> GPMTSQKLVRLPGLIDVHVHLREPGGTHKEDFASGTAAALAGGITMVCAMPNTRPPIIDGPALALAQKLAEAGARCDFALFLGASSENAGTLGTVAGSAAGLKLYLNETTSELRLDSVVQWMEHFETWPSHLPIVAHAEQQTVAAVLMVAQLTQRSVHICHVARKEEILLIKAAKARGLPVTCEVAPHHLFLSHDDLERLGPGKGEVRPELGSRQDVEALWENMAVIDCFASDHAPHTLEEKCGSRPPPGFPGLETMLPLLLTAVSEGRLSLDDLLQRLHHNPRRIFHLPPQEDTYVEVDLEHEWTIPSHMPFSKAHWTPFEGQKVKGTVRRVVLRGEVAYIDGQVLVPPGYGQDVRK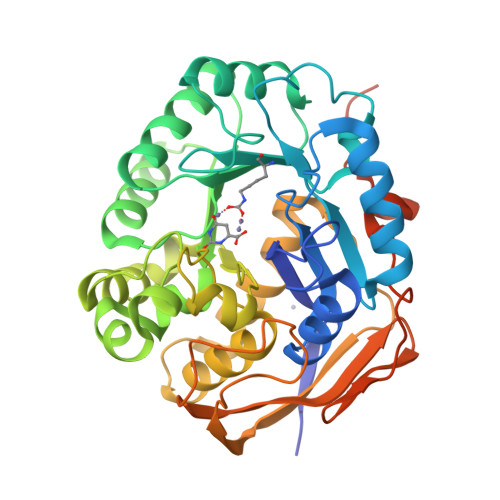WPQGAVPQLPPSAPATSEMTTTPERPRRGIPGLPD The AMP-forming acetyl-CoA synthetase is regulated by lysine acetylation both in bacteria and eukaryotes. AMP-forming acetyl-CoA synthetases catalyse the ATP-dependent formation of acetyl-CoA from acetate and coenzyme A in two half-reactions. In the first half-reaction, acetyl-CoA synthetase activates acetate using ATP to form acetyl-AMP under the release of pyrophosphate PPi (adenylation reaction). In the second half-reaction, the thioester acetyl-CoA is generated from the mixed anhydride acetyl-AMP and CoA releasing AMP (thioesterification/thioester-formation).

Crystal structures of AcsA from Chloroflexota bacterium in the apo form and in complex with acetyl-adenosine-5′-monophosphate (acetyl-AMP) support the flexible C-terminal domain adopting different conformations. Our structural data on Chloroflexota bacterium AcsA in complex with acetyl-AMP, the product of the first half-reaction, shows that in this thioester-forming conformation, K624 (corresponds to K549 of B. subtilis AcsA and K609 of S. enterica Acs) is exposed. In this conformation, the acetylated/non-acetylated lysine (B. subtilis AcsA: K549) will be accessible for a deacetylase or an acetyltransferase to be deacetylated or acetylated. In contrast to the previous report, at least in this case product formation of the adenylation reaction alone, i.e. binding of acetyl-AMP, rather than CoA binding is sufficient to stabilize the thioester-forming conformation, which is capable of subsequent CoA binding. We show that AlphaFold2 is a powerful tool to generate initial models, however, as shown by the experimentally determined structure of acetyl-AMP bound AcsA of Chloroflexota bacterium, AlphaFold2 is not able to predict all conformations with various ligands or combinations thereof adapted by AcsA. Notably, we found in the apo structure and in the acetyl-AMP-bound AcsA structure of the Chloroflexota bacterium a phosphorylated histidine residue, i.e. His476, in the C-terminal domain. This histidine is not conserved amongst other members of AMP-forming acetyl-CoA synthetases.

>[4x]MAHHHHHHVGTSSNLSFEHTDNILIEERLFPPPEDIVKNANITAYMKSKGFDDYEAFYRWSLANRFEFWNDMAKELHWFEPWKSTFEWTDKPFFKWFTDGKFNIAYNCLDRYMGTPIEDKVAFYWEGDDGSSRAYTYKEMYVLTNRVAKVLQNQGVKKGDRVAIYMPMIPEMAASVLACARLGAPHMVVFGGFAASSLRDRMNDCDAKVLITADGGYRGGKVIELKKIADEAVAETPTIEKVFVQRHTGFEVPMAEGRDVYLDVLLNDIPEDTVVPCEPVDSEDMLYILYTSGSTGKPKGVVHVHGGYAVGCYATTKFVFDIKPSDVFWCTADIGWVTGHSYTIYGPMMNAASIVLFEGIPTYPAADRFWSIVEKYKVNIIYTAPTAIRSLMRFGEELPARHDLSSLRILGTVGEPINPEAWMWYRKNIGHNELPIMDTWWQTETGMILISPTPILPLKPGSASRPLPTIEADVVNKDGKPVGPEHGGFLIIRHPWPAQMRTIFGDPDRYKTYWETIPDVYFAGDAATMDKMGYFRIQGRVDDVIKVSGHRLGSMEIESSLVSHPAVAEAAAIGKPDEVKGEHVKVFVILRNGVEPTESLAVELKRHVRTLVGPLATPDELEFVTSLPKTRSGKIMRRVVRARELGEPVGDITTLDV> VQLKGRDLLTLKNFTGEEIKYMLWLSADLKFRIKQKGEYLPLLQGKSLGMIFEKRSTRTRLSTETGFALLGGHPCFLTTQDIHLGVNESLTDTARVLSSMADAVLARVYKQSDLETLAKEASIPVINGLSDLYHPIQILADYLTLQEHYSSL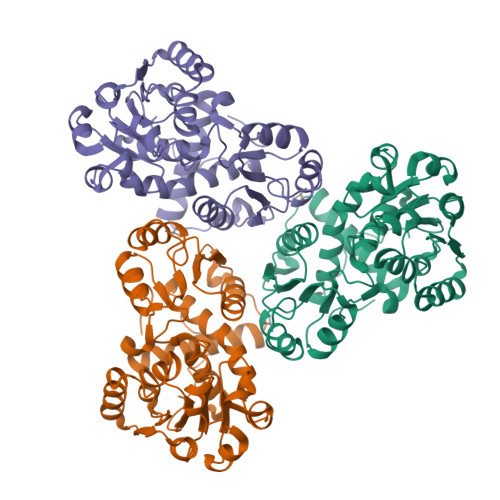KGLTLSWIGDGNNILHSIMMSAAKFGMHLQAATPKGYEPDASVTKLAEQYAKENGTKLLLTNDPLEAAHGGNVLITDTWISMGREEEKKKRLQAFQGYQVNSKTAKVAASAWTFLHCLPRKPEEVDDDVFYSPRSLVFPEAENRKWTIMAVMVSLLTDYSPQLQKPKF>[4x]MSNCQYKIYPPLGIARVGNGPAIKPLSLSTPEVPWAHLYDTNVQYLVTQQELEQLLEEAFGGNVINEISQIKTKLDERKAEKFKQEEIETITGLLGLSHLVPQQQLSRSLDNLELKSTKDSDDIVQQIKGALLKVLSDHYLHAVKKQAQNFYIYKCDEQGNPVEKLKLTDGDKVTWRVEVANKKSFWYDYNN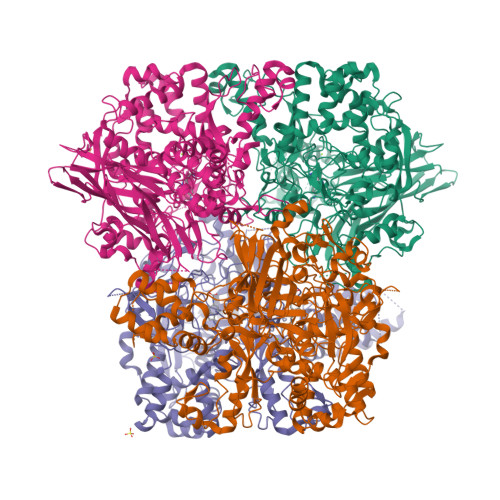ALDLSLHTQGSGNLSKNVSKHRLAPAMTAKRRNPNVITNSLRKQLVISSQGSVSSDNNTQVPLRGKFPANEPDTNNRLSDLLNLQERHNVLQGSIECDNEGVLRFYAGNGISQALSPSSLNTDFADNSNWFDDICDGRVTAVVELKNGDTFEIQDEQSSAWVATTPPDYAPQIEPIVTMYDMVSGAALKEQDLDNLTTQFSDVFPILYRLYRMQWVNQADFTDNAVNTQIRELNSELGFAQLLDNSASAKSLREGIFNQFRNPLFDQDIDVDDPGQSSNEWVSNSRIIPSKDETNIAAKPATSSLKLPFYPNDGIDYPGSPVQWFAIPPFMYQHLQNWAAGDFSVTQVEKESANTIEELGLFYSEQFKNSPNSALLCARGALDALYGGGFHPGVELTWPMRHNLIYSQNDYVSSVTPEINLLGLREFRLKQDLQGLNSPNMYQDFGHVIAVDNVTASIDPNSDAAWLWRSTPGDLTKWMGIPWQSDAASCQAVYTPEDFPIPSWXAANLPVHVLPLARYNKFKDSQSADLPEINGMTHSIAQGMSEETFEHLRLEQFSQRLDWLHTADLGFVGFHAEGGYTNGLIQMVSQWKNMAMVMARPVENPGSSGIPNVVYVAYSQADKD>QRCGEQGSGMECPNNLCCSQYGYCGMGGDYCGKGCQNGACWTSKRCGSQAGGKTCPNNHCCSQYGHCGFGAEYCGAGCQGGPCRADIKCGSQAGGKLCPNNLCCSQWGYCGLGSEFCGEGCQNGACST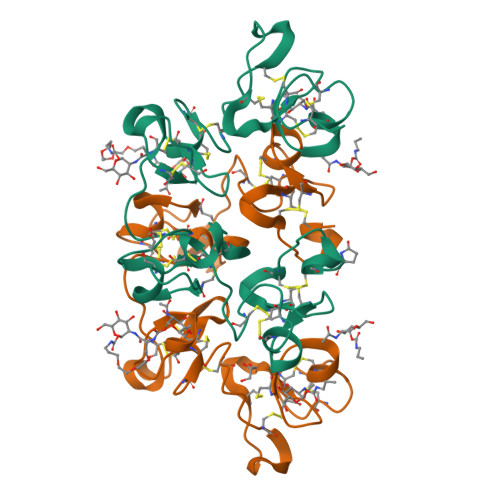DKPCGKDAGGRVCTNNYCCSKWGSCGIGPGYCGAGCQSGGCDG[2x]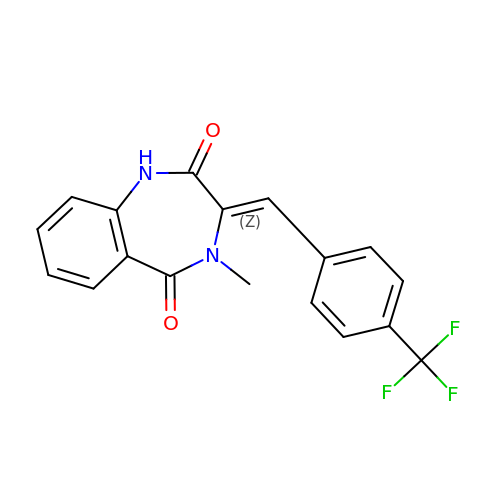(3~{Z})-4-methyl-3-[[4-(trifluoromethyl)phenyl]methylidene]-1~{H}-1,4-benzodiazepine-2,5-dione | C18 H13 F3 N2 O2 | NVEJUUHKRHQWHW-GDNBJRDFSA-N>[2x]RDGERTVYCNVHK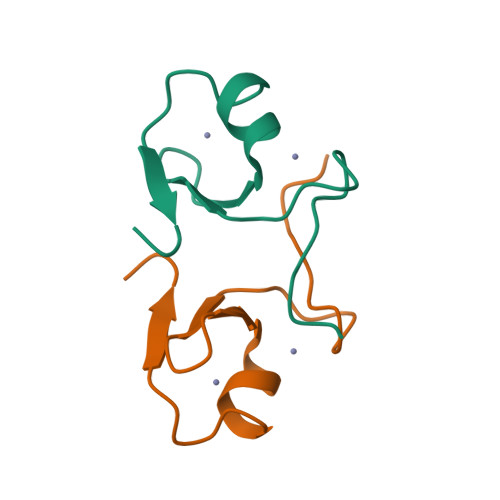HEPLVLFCESCDTLTCRDCQLNAHKDHQYQFLEDAVR> MAASYEEERDIQKNYWIEHSADLTVEAMMLDSRASDLDKEERPEVLSLLPPYEGKSVLELGAGIGRFTGELAQKAGELIALDFIDNVIKKNESINGHYKNVKFMCADVTSPDLKITDGSLDLIFSNWLLMYLSDKEVELLAERMVGWIKVGGYIFFRESCFHQSGDSKRKSNPTHYREPRFYSKVFQECQTRDAAGNSFELSMIGCKCIGAYVKNKKNQNQICWIWQKVSSENDRGFQRFLDNVQYKSSGILRYERVFGQGFVSTGGL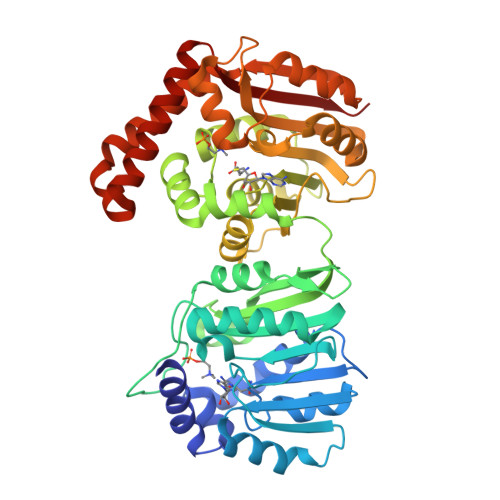ETTKEFVEKMNLKPGQKVLDVGCGIGGGDFYMAEKFDVHVVGIDLSVNMISFALERAIGLSCSVEFEVADCTTKHYPDNSFDVIYSRDTILHIQDKPALFRTFFKWLKPGGKVLISDYCRSPKTPSAEFSEYIKQRGYDLHDVQAYGQMLKDAGFTDVIAEDRTDQFMQVLKRELDRVEKEKEKFISDFSKEDYDDIVGGWKSKLERCASDEQKWGLFIANKN>DALHDQASALFKPIPEQVTELRGQPISEQQRELGKKLFFDPRLSRSHVLSCNTCHNVGTGGADNVPTSVGHGWQK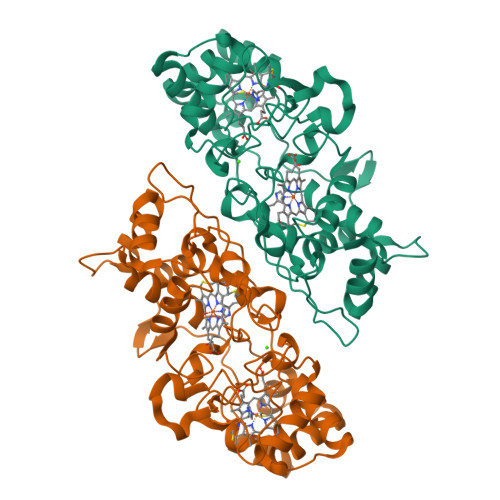GPRNSPTVFNAVFNAAQFWDGRAKDLGEQAKGPIQNSVEMHSTPQLVEQTLGSIPEYVDAFRKAFPKAGKPVSFDNMALAIEAYEATLVTPDSPFDLYLKGDDKALDAQQKKGLKAFMDSGCSACHNGINLGGQAYFPFGLVKKPDASVLPSGDKGRFAVTKTQSDEYVFRAAPLRNVALTAPYFHSGQVWELKDAVAIMGNAQLGKQLAPDDVENIVAFLHSLSGKQPRVEYPLLPASTETTPRPAE[2x]>[2x]GSMRICIFMARGLEGCGVTKFSLEQRDWFIKNGHEVTLVYAKDKSFTRTSSHDHKSFSIPVILAKEYDKALKLVNDCDILIINSVPATSVQEATINNYKKLLDNIKPSIRVVVYQHDHSVLSLRRNLGLEETVRRADVIFSHSDNGDFNKVLMKEWYPETVSLFDDIEEAPTVYNFQPP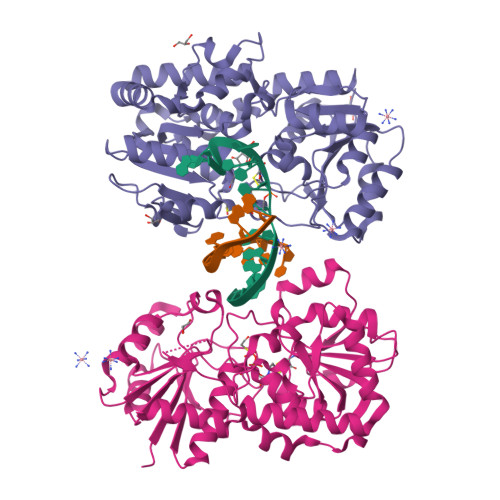MDIVKVRSTYWKDVSEINMNINRWIGRTTTWKGFYQMFDFHEKFLKPAGKSTVMEGLERSPAFIAIKEKGIPYEYYGNREIDKMNLAPNQPAQILDCYINSEMLERMSKSGFGYQLSKLNQKYLQRSLEYTHLELGACGTIPVFWKSTGENLKFRVDNTPLTSHDSGIIWFDENDMESTFERIKELSSDRALYDREREKAYEFLYQHQDSSFCFKEQFDIITK>MCSTCANVLKYYNWDPHFRLVIDPNKFLSVGFCDNPLMCCYPELLPEFGTVWDCDQSPLQIYLESILGDDEWASTYEAIDPAVPPMHWDAAGKIFQPHPGVLMHHLIGEVAKAWDPNLPMFRLEADGDGSITAPEQGTPVGGVIAEPSAQMSAAADMATGKSVDSEWEAFFSFHTSVNWSTSETQGKILFKQSLGPLLNPYLEHLAKLYVAWSGSIDVRFSISGSGVFGGKLAAIVVPPGVDPVQSTSMLQYPHVLFDARQVEPVIFSIPDLRSTLYHLMSDTDTTSLVIMVYNDLINPYANDSNSSGCIVTVETKPGADFKFHLLKPPGSMLTHGSVPSDLIPKSSSLWIGNRHWTDITDFVIRPFVFQANRHFDFNQETAGWSTPRYRPITITISEKNGAKLGIGVATDYIVPGIPDGWPDTTIPEKLTPAGDYAITNKSGNDITTAAGYDGADVIVNNTNFKGMYICGSLQRAWGDKKISNTAFITTATKVDNAIEPSNVIDMTKIAVYQDTHVGKEVQTSDDTLSLLGYTGIGEQAIGSDRDRVVRISVLPETGARGGNHPIFYKNSIKLGYVIRSIDVFNSQILHTSRQLSLNHYLLPPDSFAVYRIIDSNGSWFDIGIDSDGFSFVGVSSIGKLEFPLTASYMGIQLAKIRLASNIRSSMTKL[4x];>[4x]AVYTSEPDVRVPEDKPAKLSCSYSGFSNPRVEWKFAHGDITSLVCYKNKITASYADRVTFSHSGITFHSVTRKD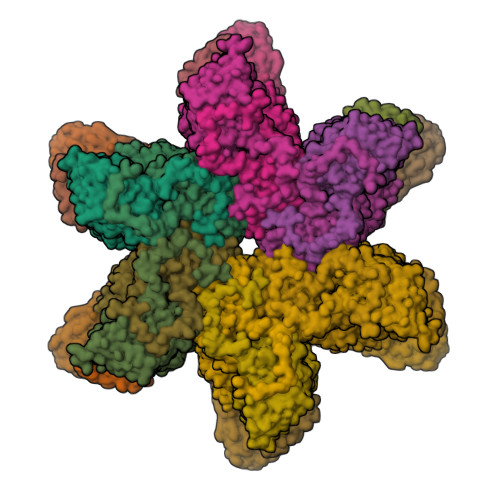TGTYTCMVSDDGGNTYGEVSVQLTVLVPPSKPTVHIPSSATIGSRAVLTCSEKDGSPPSEYYWFKDGVRMPLEPKGNRAFSNSSYSLNEKTGELVFDPVSAWDTGEYTCEAQNGYGMPMRSEAVRMEA;>MNSILGLIDTVTNTIGKAQQIELDKAALGQQRELALKRMKLDHQALNNQVEQFNKILEQRVQGPIQSVRLARAAGFRVDPYSYTDQNFYDDQLNAIRLSYRNLFKN[4x]> MNLFRKKPIQLLMKESGAKGASLRKELGAFDLTMLGIGAIIGTGIFVLTGVAAAEHAGPALVLSFILSGLACVFAALCYAEFASTVPVSGSAYTYSYATFGELIAWILGWDLILEYGVASSAVAVGWSGYFQGLLSGF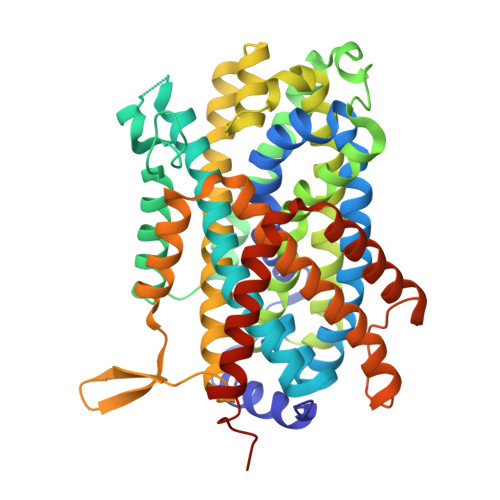GIELPKALTSAYDPAKGTFIDLPAIIIVLFITFLLNLGAKKSARFNAVIVAIKVAVVLLFLAVGVWYVKPENWTPFMPYGFSGVATGAATVFFAYIGFDAVSTAAEEVRNPQRDMPIGIIVSLLVCTLLYIAVSLVLTGIVPYEQLNVKNPVAFALNYIHQDWVAGFISLGAIAGITTVLLVMMYGQTRLFYAISRDGLLPKVFARISPTRQVPYVNTWLTGAAVAVFAGIIPLNKLAELTNIGTLFAFITVSIGVLVLRKTQPDLKRAFRVPFVPVVPILAVLFCGYLVLQLPAMTWIGFVSWLLIGLVIYFIYGRKHSELNEMARTEEKAG> SKNLILDFPQPSTDYLSFRSHFQKNFVCLENCSLQERTVTGTVKVKNVSFEKKVQIRITFDSWKNYTD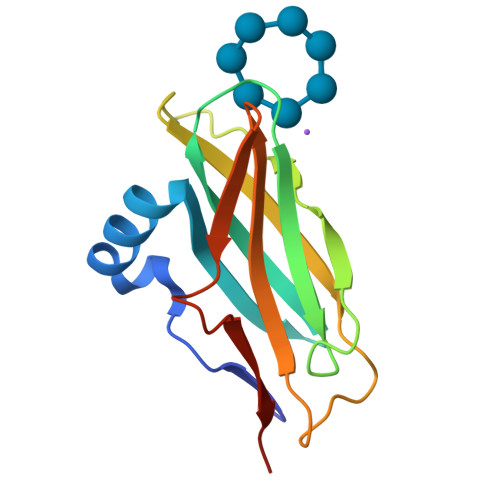VDCVYMKNVYGGTDSDTFSFAIDLPPVIPTEQKIEFCISYHANGQVFWDNNDGQNYRIVHVQWKPD>[8x]GSHMTSFLHAYFTRLHCQPLGVPTVEALRTLHLAHNCAIPFENLDVLLPREIQLDETALEEKLLYARRGGYCFELNGLFERALRDIGFNVRSLLGRVILSHPASLPPRTHRLLLVDVEDEQWIADVGFGGQTLTAPLRLQAEIAQQTPHGEYRLMQEGSTWILQFRHHEHWQSMYCFDLGVQQQSDHVMGNFWSAHWPQSHFRHHLLM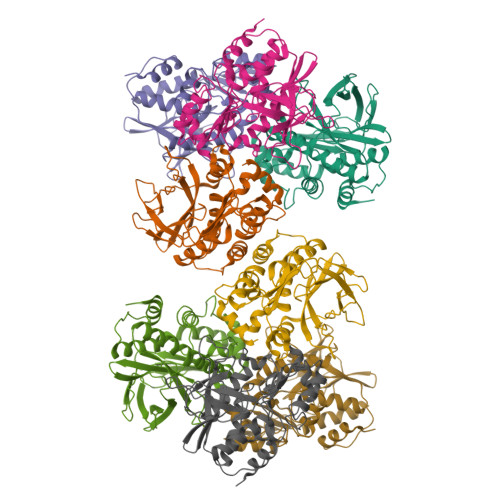CRHLPDGGKLTLTNFHFTRYHQGHAVEQVNVPDVPSLYQLLQQQFGLGVNDVKHGFTEAELAAVMAAFDTHPEAGK>GHMSGRGKKPTRTLVMTSMPSEKQNVVIQVVDKLKGFSIAPDVCETTTHVLSGKPLRTLNVLLGIARGCWVLSYDWVLWSLELGHWISEEPFELSHHFPAAPLCRSECHLSAGPYRGTLFADQPVMFVSPASSPPVAKLCELVHLCGGRVSQVPRQASIVIGPYSGKKKATVKYLSEKWVLD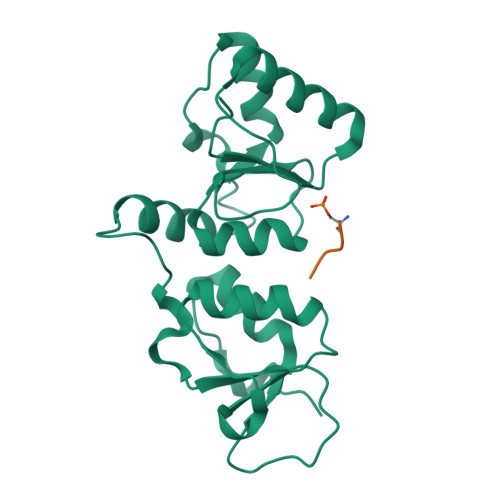SITQHKVCAPENYLLSQ[2x];>SDEF[2x]N-[(2S,3R)-4-{[(4S)-2-(2,2-dimethylpropyl)-6,6-dimethyl-4,5,6,7-tetrahydro-2H-indazol-4-yl]amino}-3-hydroxy-1-phenylbutan-2-yl]acetamide | C26 H40 N4 O2 | 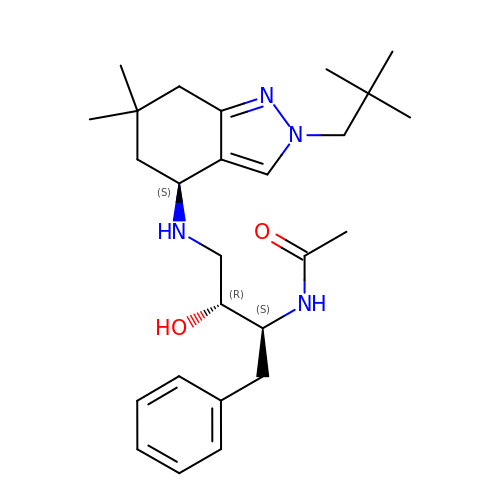RUVGZLLBYDXKFE-WPFOTENUSA-N>[2x]GGMQTNSKIYIAGHKGTAGTALVENLQKRGFNNLVLKTRQELDLVNQQAVAKFFKEEKPEYVFLTAVLPCGAANVAQRADFIYENLMIQNNVIHNSFLNNVKKLVFFGSGYMYPENAKNPLKEEYLFQGDLEYGAYSFGAAKIAGAIMCESYNIQYGTNFITLVLNNLYGTKANFDFGKSRVLPAL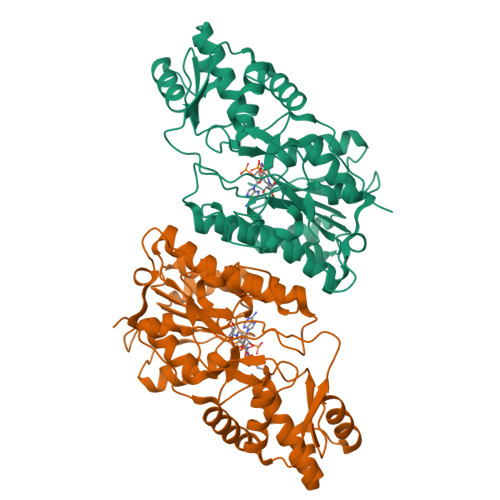LRKFHLAKLLSEGNITQILQDLKMNNFEEAKEYLHNFGISKKSVEIWGTGKVRREFIHSDDLADVAIYTMQNIDFKDLIKDRKSKNTHINIGTGIDYSIKEVALMVKNIVGFSGELVFNTSRPDSTMDRLMDCSKIHSLGWKHKIELKDGIKMMYEWYKTQN1,2-DIDECANOYL-SN-GLYCERO-3-PHOSPHOETHANOLAMINE | C25 H49 N O8 P | 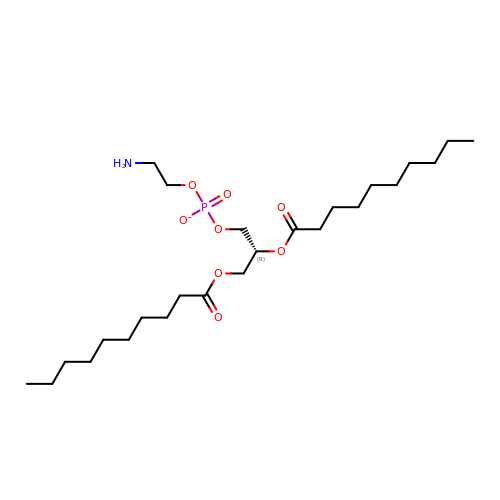KKOSJVWUOHEQKA-HSZRJFAPSA-M> MRRNRRGSPARPAARFVRPAIPSALSVALLVCTPGLATADPQTDTIAALIADVAKANQRLQDLSDEVQAEQESVNKAMVDVETARDNAAAAEDDLEVSQRAVKDANAAIAAAQHRFDTFAAATYMNGPSVSYLSASSPDEIIAT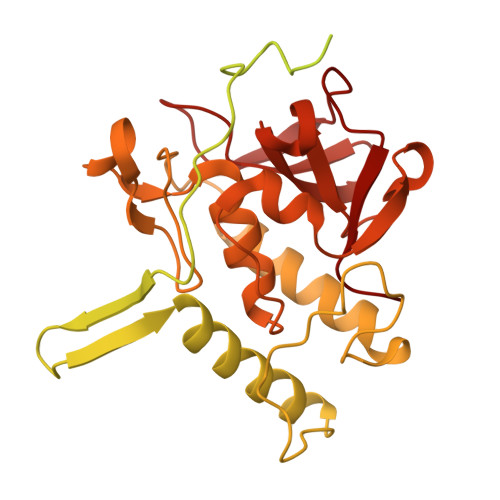VTAAKTLSASSQAVMANLQRARTERVNTESAARLAKQKADKAAADAKASQDAAVAALTETRRKFDEQREEVQRLAAERDAAQARLQAARLVAWSSEGGQGAPPFRMWDPGSGPAGGRAWDGLWDPTLPMIPSANIPGDPIAVVNQVLGISATSAQVTANMGRKFLEQLGILQPTDTGITNAPAGSAQGRIPRVYGRQASEYVIRRGMSQIGVPYSWGGGNAAGPSKGIDSGAGTVGFDCSGLVLYSFAGVGIKLPHYSGSQYNLGRKIPSSQMRRGDVIFYGPNGSQAVTIYLGNGQMLEAPDVGLKVRVAPVRTAGMTPYVVRYIEY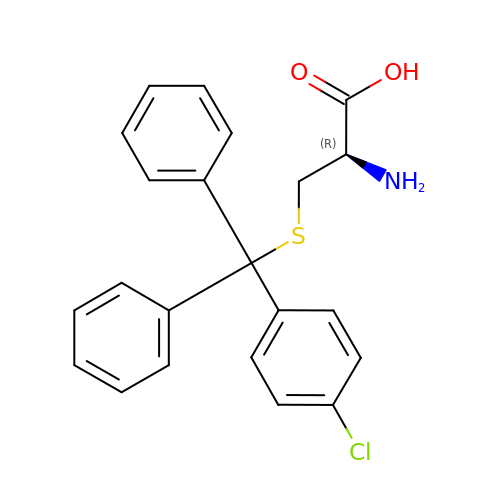(2R)-2-AMINO-3-[(4-CHLOROPHENYL)-DIPHENYL-METHYL]SULFANYL-PROPANOIC ACID | C22 H20 Cl N O2 S | BSTXYLCINUXYQF-FQEVSTJZSA-N>[2x]TEFLKPRLVDIEQVSSTHAKVTLEPLERGFGHTLGNALRRILLSSMPGCAVTEVEIDGVLHEYSTKEGVQEDILEILLNLKGLAVRVQGKDEVILTLNKSGIGPVTAADITHDGDVEIVKPQHVICHLTDENASISMRIKVQRGRGYVPASTRIHSEEDERPIGRLLVDACYSPVERIAYNVEAARVEQRTDLDKLVIEMETNGTIDPEEAIRRAATILAEQLEAFVDLRD;> YSYTEKKRIRKDFGKRPQVLDVPYLLSIQLDSFQKFIEQDPEGQYGLEAAFRSVFPIQSYSGNSELQYVSYRLGEPVFDVQECQIRGVTYSAPLRVKLRLVIYEREAPEGTVKDIKEQEVYMGEIPLMTDNGTFVINGTERVIVSQLHRSPGVFFDSDKGKTHSSGKVLYNARIIPYRGSWLDFEFDPKDNLFVRIDRRRKLPATIILRALNYTTEQILDLFFEKVIFEIRDNKLQMELVPERLRGETASFDIEANGKVYVEKGRRITARHIRQLEKDDVKLIEVPVEYIAGKVVAKDYIDESTGELICAANMELSLDLLAKLSQSGHKRIETLFTNDLDHGPYISETLRVDPTNDRLSALVEIYRMMRPGEPPTREAAESLFENLFFSEDRYDLSAVGRMKFNRSLLREEIEGSGILSKDDIIDVMKKLIDIRNGKGEVDDIDHLGNRRIRSVGEMAENQFRVGLVRVERAVKERLSLGDLDTLMPQDMINAKPISAAVKEFFGSSQLSQFMDQNNPLSEITHKRRISALGPGGLTRERAGFEVRDVHPTHYGRVCPIETPEGPNIGLINSLSVYAQTNEYGFLETPYRKVTDGVVTDEIHYLSAIEEGNYVIAQANSNLDEEGHFVEDLVTCRSKGESSLFSRDQVDYMDVSTQQVVSVGASLIPFLEHDDANRALMGANMQRQAVPTLRADKPLVGTGMERAVAVDSGVTAVAKRGGVVQYVDASRIVIKVNEDEMYPGEAGIDIYNLTKYTRSNQNTCINQMPCVSLGEPVERGDVLADGPSTDLGELALGQNMRVAFMPWNGYNFEDSILVSERVVQEDRFTTIHIQELACVSRDTKLGPEEITADIPNVGEAALSKLDESGIVYIGAEVTGGDILVGKVTPKGETQLTPEEKLLRAIFGEKASDVKDSSLRVPNGVSGTVIDVQVFTRDGVEKDKRALEIEEMQLKQAKKDLSEELQILEAGLFSRIRAVLVAGGVEAEKLDKLPRDRWLELGLTDEEKQNQLEQLAEQYDELKHEFEKKLEAKRRKITQGDDLAPGVLKIVKVYLAVKRRIQPGDKMAGRHGNKGVISKINPIEDMPYDENGTPVDIVLNPLGVPSRMNIGQILETHLGMAAKGIGDKINAMLKQQQEVAKLREFIQRAYDLGADVRQKVDLSTFSDEEVMRLAENLRKGMPIATPVFDGAKEAEIKELLKLGDLPTSGQIRLYDGRTGEQFERPVTVGYMYMLKLNHLVDDKMHARSTGSYSLVTQQPLGGKAQFGGQRFGEMEVWALEAYGAAYTLQEMLTVKSDDVNGRTKMYKNIVDGNHQMEPGMPESFNVLLKEIRSLGINIELEDE;> TEEFDAIKIALASPDMIRSWSFGEVKKPETINYRTFKPERDGLFCARIFGPVKDYECLCGKYKRLKHRGVICEKCGVEVTQTKVRRERMGHIELASPTAHIWFLKSLPSRIGLLLDMPLRDIERVLYFESYVVIEGGMTNLERQQILTEEQYLDALEEFGDEFDAKMGAEAIQALLKSMDLEQECEQLREELNETNSETKRKKLTKRIKLLEAFVQSGNKPEWMILTVLPVLPPDLRPLVPLDGGRFATSDLNDLYRRVINRNNRLKRLLDLAAPDIIVRNEKRMLQEAVDALLDNGRRGRAITGSNKRPLKSLADMIKGKQGRFRQNLLGKRVDYSGRSVITVGPYLRLHQCGLPKKMALELFKPFIYGKLELRGLATTIKAAKKMVEREEAVVWDILDEVIREHPVLLNRAPTLHRLG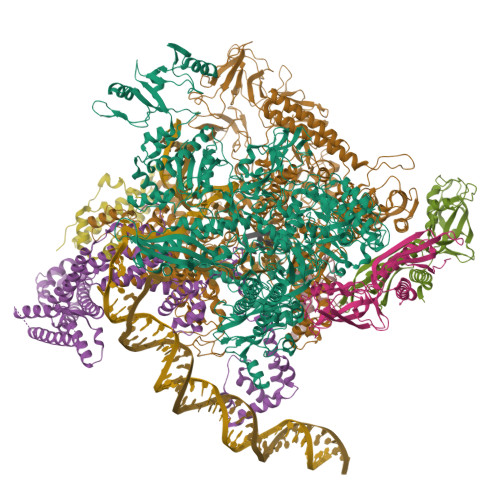IQAFEPVLIEGKAIQLHPLVCAAYNADFDGDQMAVHVPLTLEAQLEARALMMSTNNILSPANGEPIIVPSQDVVLGLYYMTRDCVNAKGEGMVLTGPKEAERLYRSGLASLHARVKVRITEYEKDANGELVAKTSLKDTTVGRAILWMIVPKGLPYSIVNQALGKKAISKMLNTCYRILGLKPTVIFADQIMYTGFAYAARSGASVGIDDMVIPEKKHEIISEAEAEVAEIQEQFQSGLVTAGERYNKVIDIWAAANDRVSKAMMDNLQTETVINRDGQEEKQVSFNSIYMMADSGARGSAAQIRQLAGMRGLMAKPDGSIIETPITANFREGLNVLQYFISTHGARKGLADTALKTANSGYLTRRLVDVAQDLVVTEDDCGTHEGIMMTPVIEGGDVKEPLRDRVLGRVTAEDVLKPGTADILVPRNTLLHEQWCDLLEENSVDAVKVRSVVSCDTDFGVCAHCYGRDLARGHIINKGEAIGVIAAQSIGEPGTQLTMRTFHIGGAASRAAAESSIQVKNKGSIKLSNVKSVVNSSGKLVITSRNTELKLIDEFGRTKESYKVPYGAVLAKGDGEQVAGGETVANWDPHTMPVITEVSGFVRFTDMIDGQTITRQTDELTGLSSLVVLDSAERTAGGKDLRPALKIVDAQGNDVLIPGTDMPAQYFLPGKAIVQLEDGVQISSGDTLARIPQESGGTKDITGGLPRVADLFEARRPKEPAILAEISGIVSFGKETKGKRRLVITPVDGSDPYEEMIPKWRQLNVFEGERVERGDVISDGPEAPHDILRLRGVHAVTRYIVNEVQDVYRLQGVKINDKHIEVIVRQMLRKATIVNAGSSDFLEGEQVEYSRVKIANRELEANGKVGATYSRDLLGITKASLATESFISAASFQETTRVLTEAAVAGKRDELRGLKENVIVGRLIPAGTGYAYHQDRMRRRAAG;> ARVTVQDAVEKIGNRFDLVLVAARRARQMQVGGKDPLVPEENDKTTVIALREIEEGLINNQILDVRERQEQQEQEA;> EIGRTTDPVRMYMREMGTVELLTREGEIDIAKRIEDGINQVQCSVAEYPEAITYLLEQYDRVEAEEARLSDLITGFVDPNAEEDLAPTATHVGSELSQEDLDDDEDEDEEDGDDDSADDDNSIDPELAREKFAELRAQYVVTRDTIKAKGRSHATAQEEILKLSEVFKQFRLVPKQFDYLVNSMRVMMDRVRTQERLIMKLCVEQCKMPKKNFITLFTGNETSDTWFNAAIAMNKPWSEKLHDVSEEVHRALQKLQQIEEETGLTIEQVKDINRRMSIGEAKARRAKKEMVEANLRLVISIAKKYTNRGLQFLDLIQEGNIGLMKAVDKFEYRRGYKFSTYATWWIRQAITRSIADQARTIRIPVHMIETINKLNRISRQMLQEMGREPTPEELAERMLMPEDKIRKVLKIAKEPISMETPIGDDEDSHLGDFIEDTTLELPLDSATTESLRAATHDVLAGLTAREAKVLRMRFGIDMNTDYTLEEVGKQFDVTRERIRQIEAKALRKLRHPSRSEVLRSFLD;> MTKITVNYTVDVKDIQPKHVRSESNPQNQNKIRRAWVLSLSDNAMEVIQNKIKSAPARHAYYEAIDREVSNKWIELMRKHTTESLNAGAKFIMTSCGERLEDDYCGNADERLIVAAQIVAETIAADFNR>[4x]GRKERERLEEKLEDANERIAELVKLEERQRIARDLEDTLGQKLSLIGLKSDLARKLIYKDPEQAARELKSVQQTARTSLNEVRKIVSSMKGIRLKDELINIKQILEAADIMFIYEEEKWPENISLLNENILSMCLKEAVTNVVKHSQAKTCRVDIQQLWKEVVITVSDDGTFKGEENSFSKGHGLLGMRERLEFANGSLHIDTENGTKLTMAIPNNSK;>[2x]GSGSMISIFIAEDQQMLLGALGSLLNLEDDMEVVGKGTTGQDAVDFVKKRQPDVCIMDIEMPGKTGLEAAEELKDTGCKIIILTTFARPGYFQRAIKAGVKGYLLKDSPSEELANAIRSVMNGKRIYAPELMEDLYSEA

The simplest TCSs comprise a sensory histidine kinase (HK) and a response regulator (RR) component. To address this question we have used the TCS DesK-DesR from B. subtilis as a model. We had previously shown that the HK DesK, a member of the HisKA_3 family, undergoes important conformational changes to switch between phosphatase- and phosphotransfer-competent states. We now report the crystal structures of the DesKC:DesR complex, trapped in the phosphatase and the phosphotransferase functional states.

One using the phosphatase-constitutive mutant DesKCSTAB, and the other with DesKCH188E carrying a phosphomimetic substitution, both in complex with the REC domain of DesR. (D) Cartoon representation of the DesKCH188E:DesR-REC (phosphotransferase) complex, along two orthogonal views (left and right subpanels). Note best fitting with a one dimer DesKCH188E (chains AB) to one monomer DesR-REC (chain C) model. The structures show the RR REC domain adopting identical conformations in both phosphatase and phosphotransferase complexes, presenting active- and inactive–like features in different regions of the protein, arranging the RR’s active site for phosphoryl group migration. The β4α4 loop in DesR plays a key role in these controls, remodeling its configuration in concert with DesK-association. This loop, acting as a phosphate lid, is open in the phosphotransferase complex, enabling the transfer reaction. Binding to unphosphorylated RR positions the P~His188(HK) into a suitable orientation for phosphoryl-transfer to occur through a loose (dissociative) nucleophilic substitution. Taking into account that phosphotransfer is a nucleophilic substitution at phosphorus, the reaction coordinate distance (i.e. between phosphorus and the entering atom, before the transfer reaction has begun) strongly suggests that P~DesK→DesR phosphotransfer occurs through a largely dissociative, or ‘loose’ mechanism: a reaction coordinate distance of ≥4.9 Å provides room for a fully dissociated metaphosphate intermediate. The small number of interactions and low surface complementarity that we observe in the several DesKC:DesR complexes are consistent with the observed ‘slippery’ nature of the protein:protein interface, displaying significant shifts in the relative positions of both partners. Further supporting that this ensemble of conformations is functionally relevant, molecular dynamics simulations of the phosphotransferase complex recapitulated the gliding shifts of one partner with respect to the other, reaching the different arrangements observed in the crystal structures at different moments of the simulations.>QRWVQFMKEAGQGSRDMWRAYSDMKKANWKNSDKYFHARGNYDAARRGPGGAWAAKVISDAREAVQKFTGHGAEDSRADQFANEWGRSGKDPNHF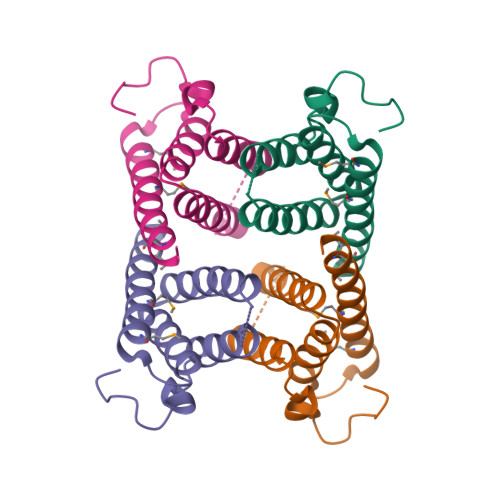RPAGLPKRY[2x]> MSLVNGRRRTAASVVALTAALTALAALCAPAQAQDTKATSKAAEAAKPDAGTLRVCAAEQPPLSMKDGSGLENRIATTVAEAMGRKA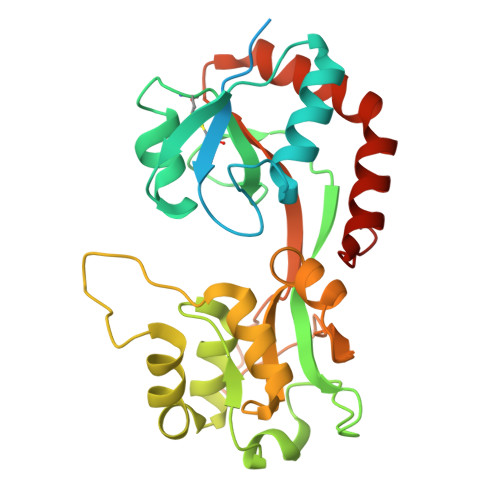QFVWLGKPAIYLVRDGLEKKTCDVVIGLDADDPRVLTSKPYYRSGYVFLTRADKDLDIKSWSDPRLKEVSHMVVGFGTPGEAMLKDIGRYEEDMAYLYSLVNFRAPRNQYTQIDPARMVSEVATGKAEVGVAFGPDVARYVRDSSTKLRMTPVPDDTQASDGRKMPQSFDQAMGVRKDDTALKAEIDAALEKAKPKIEAILKEEGVPVLPVSN6-{[(3R,4R)-4-(2-{[(2R)-2-fluoro-2-(3-fluorophenyl)ethyl]amino}ethoxy)pyrrolidin-3-yl]methyl}-4-methylpyridin-2-amine 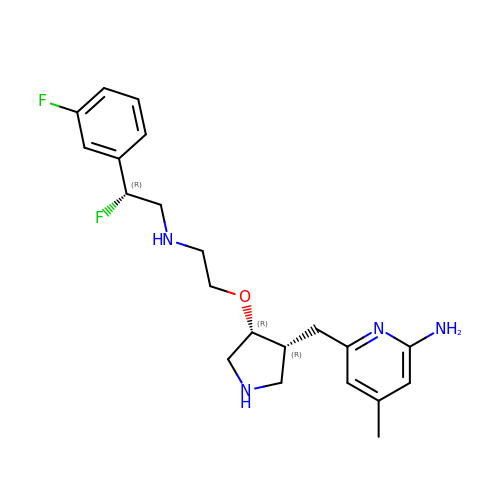| C21 H28 F2 N4 O | NOLWAWWUERSXHH-UXPWSPDFSA-N C‐reactive protein (CRP) is an evolutionarily highly conserved, acute phase protein that is synthesized in the liver under the regulation of the cytokine interleukin 6 (IL6) and circulates as a disc‐shaped homo‐pentamer (pCRP) (Zeller et al, 2022). We recently identified a novel mechanism that leads to a conformational change from the native, functionally relatively inert, pentameric CRP (pCRP) structure to a pentameric CRP intermediate (pCRP*) and ultimately to the monomeric CRP (mCRP) form, both exhibiting highly pro‐inflammatory effects. This transition in the inflammatory profile of CRP is mediated by binding of pCRP to activated/damaged cell membranes via exposed phosphocholine lipid head groups. The PC, PS, and PE head groups are known to bind to a shallow groove containing two calcium cations located on one face of the monomeric subunit of pCRP; hence, there are five PC/PE binding pockets on the same face of the CRP pentamer (i.e., the B‐face).

As proof‐of‐concept we present the data for a tool compound C10M, (3‐(dibutylamino)propyl)phosphonic acid, a monovalent CRP inhibitor with a molecular weight of just 250 Da. The asymmetric unit consisted of four CRP pentamers with the A‐faces stacked against each other. All of the pCRP monomers within the asymmetric unit had a C10M molecule bound. The location of the C10M molecules confirmed that the tool compound binds to the PC/PE binding pocket, with the phosphonate moiety being the main mediator of the interaction with pCRP via the calcium cations (Fig 1C through E). Residues Asn 61 and Gln 150 are in hydrogen bonding distance of oxygen atoms of the C10M phosphonate moiety, as observed in the PC:pCRP complex (Table EV1). In contrast to the positively charged quaternary amine of PC, which interacts with Glu 81 via a salt bridge, the tertiary amine of C10M appears to form hydrogen bonds with Glu 81 (Table EV1). The n‐butyl amine substituents of C10M make numerous hydrophobic contacts with pCRP residues (a full list of putative interacting pCRP residues is given in Table EV1). The C10M:pCRP complex retains the pentameric shape of circulating pCRP and, apart from the occupied PC/PE binding pocket, the remainder of the B‐face is available for partner proteins to interact. The A‐face of the C10M:pCRP complex is unhindered, hence proteins which usually interact with the A‐face of circulating pCRP should be unaffected by the bound C10M.

>[20x]QTDMSRKAFVFPKESDTSYVSLKAPLTKPLKAFTVCLHFYTELSSTRGYSIFSYATKRQDNEILIFWSKDIGYSFTVGGSEILFEVPEVTVAPVHICTSWESASGIVEFWVDGKPRVRKSLKKGYTVGAEASIILGQEQDSFGGNFEGSQSLVGDIGNVNMWDFVLSPDEINTIYLGGPFSPNVLNWRALKYEVQGEVFTKPQLWP> MAVNNNSISPAQQAQADKRARDAAAAKRKQDTEVSNAKSREDIQYTMFVSGLRRGRLNEFERKNRTDDLAILFDSVTT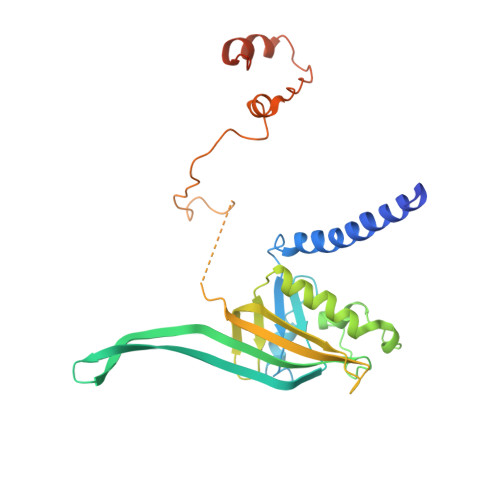HTYTKDYNKSSYAVESKAKASDHVTTQDGKFTFSGTVTDSPYLIDPRNMIDRDTDKENPMLARRPAKAIEILELIADSHQLVTLVTEDNILSNYVITSFQVDRSSEAGSSINVQVTLEEFRFKMVNKTVMARTSDPKKAKNANTGTKQTAEDGAVDDSAKQKRQTPYIGKNAETKERWENAAIGTTDFSGKPGAKLPFDPSDLMRK> MAQVQPWVDEDLKDSTEDLQVEEDAEEWQEA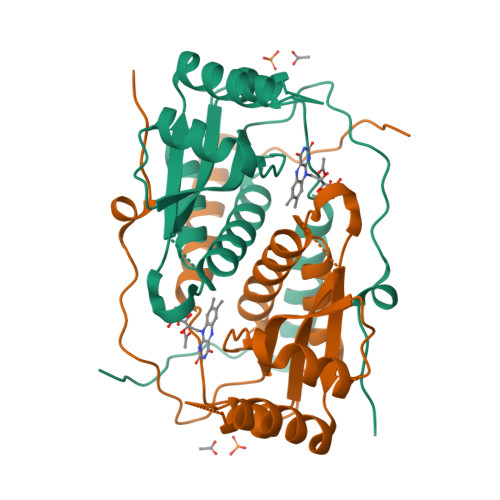EESVEHIPFSHTRYPEQEMRMRSQEFYELLNKRRSVRFISSEHVPMEVIENVIKAAGTAPSGAHTEPWTFVVVKDPDMKHKIREIIEEEEEINYMKRMGKRWVTDLKKLRTNWIKEYLDTAPVLILIFKQVHGFAANGKKKVHYYNEISVSIACGLLLAALQNAGLVTVTTTPLNCGPRLRVLLGRPSHEKLLVLLPVGYPSRDATVPDLKRKALDQIMVTVHHHHHH> SSSHHYSH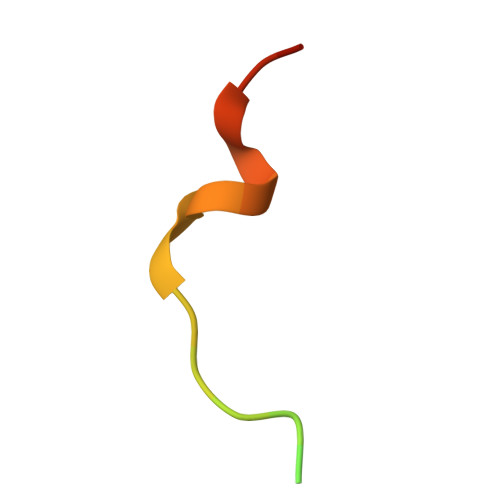PGGGGEQLAINELISDG4-O-sulfo-alpha-D-glucopyranose 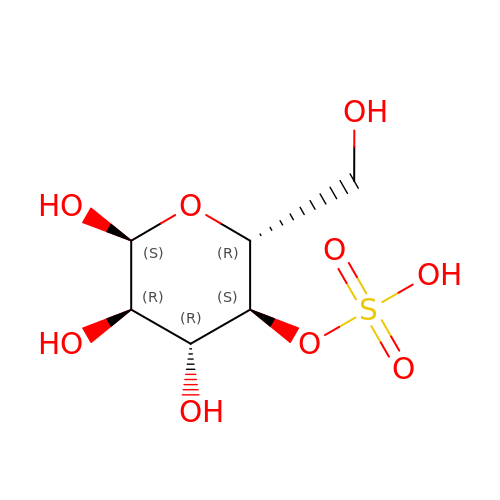| C6 H12 O9 S | LOTQRUGOUKUSEY-UKFBFLRUSA-N>GPYASLTEIEHLVQSVCKSYRETCQLRLEDLLRQRSNIFS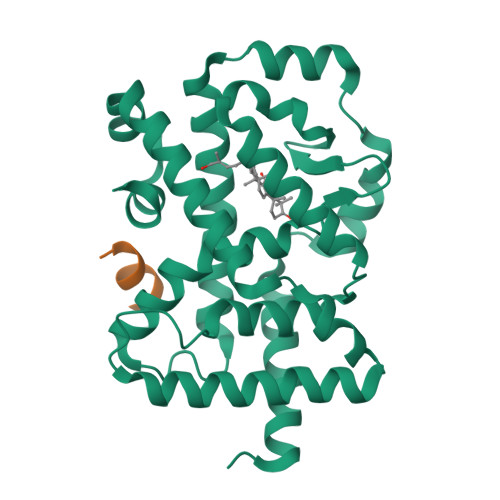REEVTGYQRKSMWEMWERCAHHLTEAIQYVVEFAKRLSGFMELCQNDQIVLLKAGAMEVVLVRMCRAYNADNRTVFFEGKYGGMELFRALGCSELISSIFDFSHSLSALHFSEDEIALYTALVLINAHRPGLQEKRKVEQLQYNLELAFHHHLSKTHRQSILAKLPPKGKLRSLCSQHVERLQIFQHLHPIVVQAAFPPLYKELFSTETESPVGLSK[4x];>NSHQKVTLLQLLLGHKNEEN[4x]>[15x]PSLSKEAALVHEALVARGLETP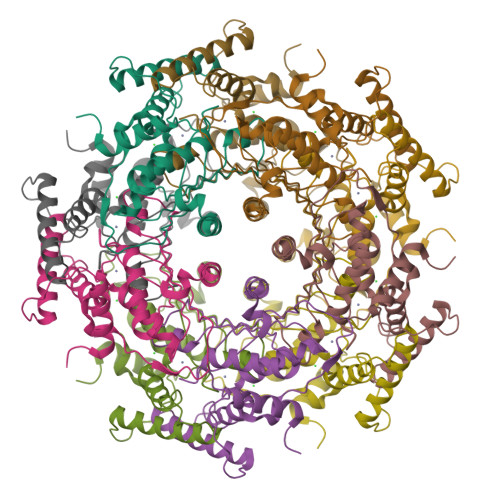LRPPVHEMDNETRKSLIAGHMTEIMQLLNLDLADDSLMETPHRIAKMYVDEIFSGLDYANFPKITLIENKMKVDEMVTVRDITLTSTCEHHFVTIDGKATVAYIPKDSVIGLSKINRIVQFFAQRPQVQERLTQQILIALQTLLGTNNVAVSIDAVHYCVKARGIRDATSATTTTSLGGLFKSSQNTRHEFLRAVRHHN> AQTHALSNAAVMDLQSRWENMPSTEQQDIVSKLSERQKLPWAQLTEPEKQAVWYISYGEWGPRRPVLNKGDSSFIAKGVAAGLLFSVGLFAVVRMAGGQDAKTMNKE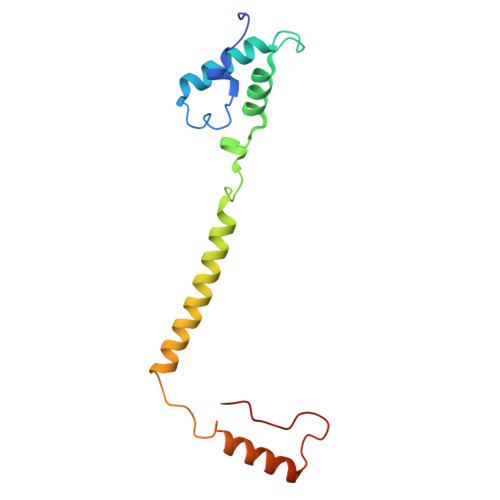WQLKSDEYLKSKNANPWGGYSQVQSK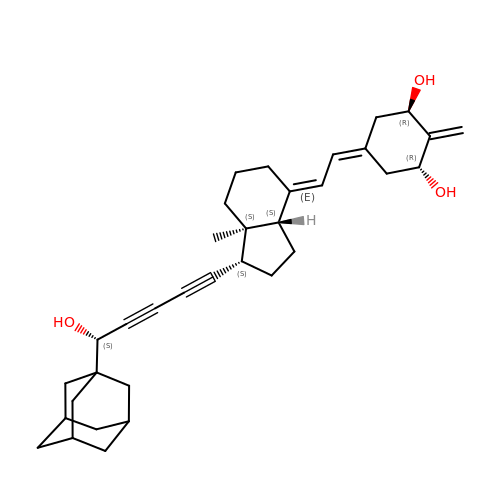(1R,3R,7E,17beta)-17-{(5S)-5-hydroxy-5-[(3R,5R,7R)-tricyclo[3.3.1.1~3,7~]dec-1-yl]penta-1,3-diyn-1-yl}-2-methylidene-9,10-secoestra-5,7-diene-1,3-diol | C34 H44 O3 | BFGRTJZGAMDLML-XMEPBAHGSA-N> LDNVATYAGQFNQDYLSGMAANMSGTFGGANMPNL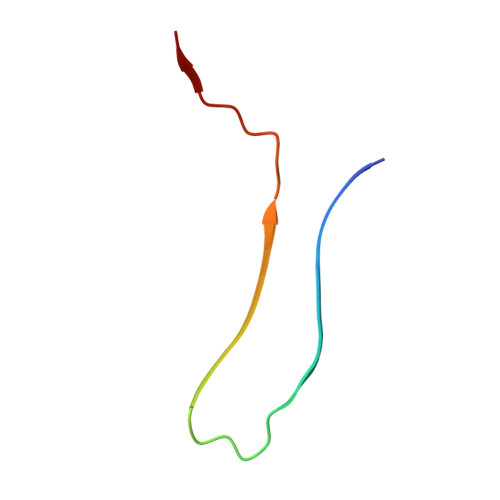Y> MTTLVLDNGAYNAKIGYSHENVSVIPNCQFRSKTARLKTFTANQIDEIKDPSGLFYILPFQKGYLVNWDVQRQVWDYLFGKEMYQVDFLDTNIIITEPY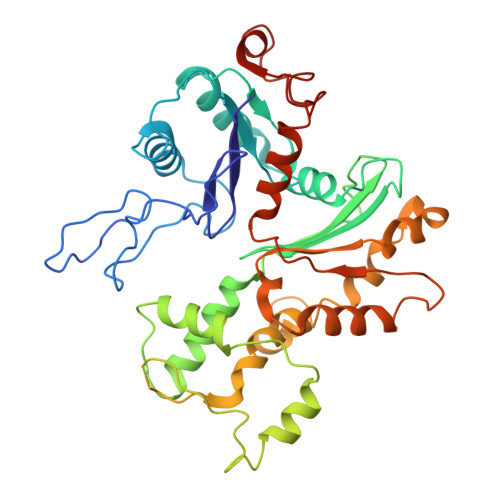FNFTSIQESMNEILFEEYQFQAVLRVNAGALSAHRYFRDNPSELCCIIVDSGYSFTHIVPYCRSKKKKEAIIRINVGGKLLTNHLKEIISYRQLHVMDETHVINQVKEDVCYVSQDFYRDMDIAKLKGEENTVMIDYVLPDFSTIKKGFCKPREEMVLSGKYKSGEQILRLANERFAVPEILFNPSDIGIQEMGIPEAIVYSIQNLPEEMQPHFFKNIVLTGGNSLFPGFRDRVYSEVRCLTPTDYDVSVVLPENPITYAWEGGKLISENDDFEDMVVTREDYEENGHSVCEEKFDI> MAEDPDPTEYLYISMEQKRKDQTKPYDGKKMVWVADEKEGYLLGLIKSTQGDICTVDIEGQESRQVKKDLLQQVNPPKYEKCEDMSNLTYLNDASVLHNLKQRYYANLIYTYSGLFCVAINPYKRFPIYTNRTVQIYKGRRRTEVPPHLFAISDGAYSAMLANRENQSMLITGESGAGKTENTKKVIAYYANVGAATPKPGKEAPTKEKKATLEDQVVQTNPVLEAFGNAKTVRNDNSSRFGKFIRIHFGPMGKLAGADIETYLLEKARVISQQTLERSYHIFYQLMSGGIENLKADLLLSDDIYDYHFVSQGKIEIPGVDDAEELRLTDTAFDILGFSHEYKTDVYKITASCMHLGEMKFKQRPREEQAEADGTEEGERVAHLLGVNAADLYKNLVKPKIKVGNEMVTQGRNATQVSYSVGGLAKAMFDRTFKWLVKRLNETLDTKQKRQYFIGVLDIAGFEIFDYNGFEQLCINFTNEKLQQFFNHHMFVLEQEEYKREGIDWVFIDFGLDLAACIELIEKPMGILSILEEESMFPKATDKSFQDKLNANHLGKSPNFVKPKPPKPGQQEAHFSIAHYAGTVPYNITGWLEKNKDPVNDTVVDQFKKGSNKLVQEIFEDHPGLGAEEKGGGGKGGGGRKKGASFQTVSALYREQLNRLMASLHSTQPHFVRCIIPNELKQPGVIDSGLVMHQLTCNGVLEGIRICRKGFPNRMVYPDFKQRYTILAASAVPKGFVDAKKVTEAVLGAIQLDANDYRLGNTKVFFRAGVLGRLEEMRDDRLGKIV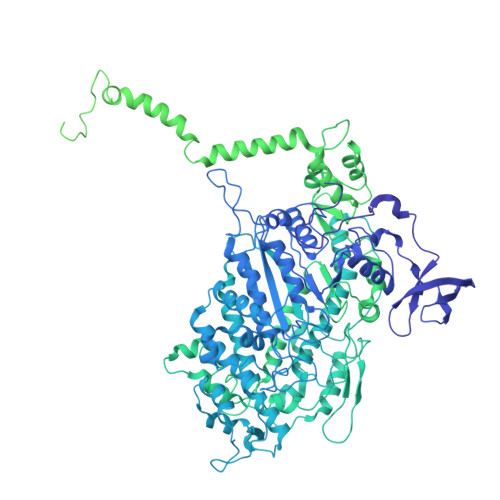TWLQAWIRWYLSKKEFKKLQEQRVALLVIQRNLRKFLTLRNWLWYKLYIKVKPLLTMAKVEDELKALEEKLKKALESLEKEEKVRKDIEVQNVKLLQEKNDLFLQLESERSGAGDVEERLTKAISMKNDLEGQVQELQERLSREEDAHSNLSSVRKKLDGEISNLKKEIEDLQLVIQKTEQDKAAKDHQIRNLNDEIAHQDELINKLNREKKQMQEMGQKTGEDLQATEDKLNHMNKVKAKLEQTLDELEDSLEREKKLRGDVEKTKRKVEGDLKLAQEAVADLEKNKKELEQALQRKEKEMASLSAKLEDEQGLVAKLQKQIKELQARIEELEEELEAERQARAKAEKQRADLAREIEELSERLEEAGGATSAQVELNKRREAEMAKLRRDLEESNIQHEQTLANLRKKHNDVVAELSEQIDQLNKHKARLEKEKAQMKGELDDVRSSVDHVNKEKANAEKQAKQLEMQLTELQGKMDEAHRSLGDFDAAKKRLTVENTELTRQLEDAESQVSQLSKLKTSLQTQLEDTKRMADEESRERATAMGKFRSVEHDLDSLREQIDEEQEGKADLQRQLSKANAEVQLWRSKYESEGLARLEELEESKRKLDAKLQEAMETIDQLNSKTSGLEKTKSRLQGELEDMTIEVEKANALASAMEKKQKSFDRIISEWKQKVDDLALELDASQKECRNYSTEVFKLRSQYEESQEHYESVKRENKNLQDEIKDLVDQLGEGGRSVHELEKARKRLELEKEELQAALEEAEAALEQEENKVLRAQLELSQVRQEIDRRLQEKEEEFENTRKNHQRAIDSMQASLEAEAKGKAEALRMKKKLESDINELEIALDHSNKANAEAQKNIKKYQIQLKETQQALEEEQRARDEVREQYAMSERRCNAMHGELEESRQLLEQADRARRAADSELAELHENVNELSAQNSSLSMAKRKLEGEMQALHADLDEMLNEAKSSEEKAKKAMVDAARLADELRAEQEHAQQQEKMRKAMEGQIKELQVRLDEAEAAALKGGKKIIQKLEQKVRELETELDNEQRRHSEAAKNVRRSERRVKELQFQAEEDRKNQERMQDLVDKLQQKIKTYKRQIEEAEEIAALNLAKFRKVQQELEDAEERADMAENVAAKLRAKNRSSASVGRAMSPIPMGKPGRPKSKIDEE3'-[(2R)-4-(2,4-diamino-6-ethylpyrimidin-5-yl)but-3-yn-2-yl]-5'-methoxy[1,1'-biphenyl]-4-carboxylic acid | C24 H24 N4 O3 | 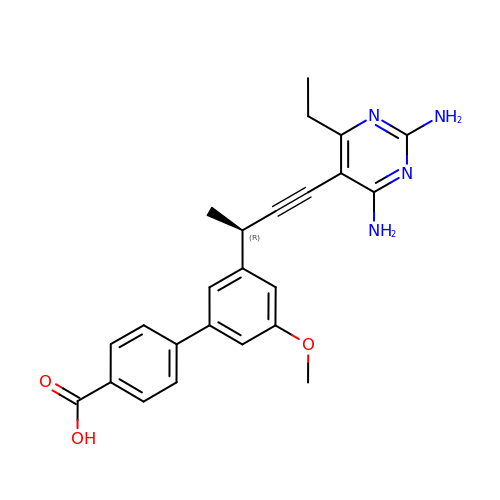OKJCHFXBCVXSIZ-AWEZNQCLSA-N> GPNVCAVQKVIGTNRKYFTNCKQWYQRKICGKSTVISYECCPGYEKVPGEKGCPAALPLSNLYETLGVVGSTTTQLYTDHTEKLRPEMEGPGSFTIFAPSNEAWASLPAEVLDSLVSNVNIELLNALRYHMVGRRVLTDELKHGMTLTSMYQNSNIQIHHYPNGIVTVNCARLLKADHHATNGVVHLIDKVISTITNNIQQIIEIEDTFETLRAAVAASGLNTMLEGNGQYTLLAPTNEAFEKIPSETLNRILGDPEALRDLLNNHILKSAMCAEAIVAGLSVETLEGTTLEVGCSGDMLTINGKAIISNKDILATNGVIHYIDELLIPDSAKTLFELAAESDVSTAIDLFRQAGLGNHLSGSERLTLLAPLNSVFKDGTPPIDAHTRNLLRNHIIKDQLASKYLYHGQTLETLGGKKLRVFVYRNSLCIENSCIAAHDKRGRYGTLFTMDRVLTPPMGTVMDVLKGDNRFSMLVAAIQSAGLTETLNREGVYTVFAPTNEAFRALPPRERSRLLGDAKELANILKYHIGDEILVSGGIGALVRLKSLQGDKLEVSLKNNVVSVNKEPVAEPDIMATNGVVHVITNVLHH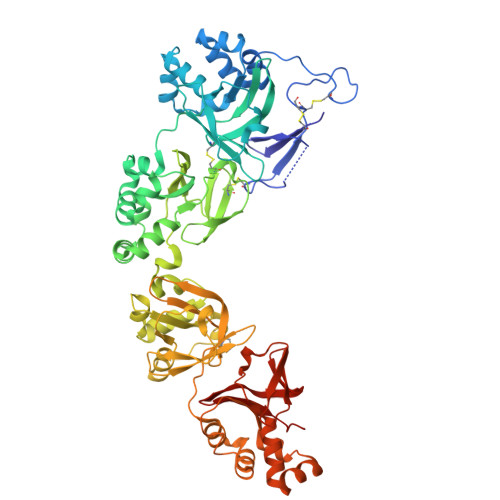HHHH> KFSAKRLPSTRLGTFLENRVNDFLRRQNHPESGEVTVRVVHASDKTVEVKPGMKARFVDSGEMAESFPYRTKALFAFEEIDGVDLCFFGMHVQEYGSDCPPPNQRRVYISYLDSVHFFRPKCLRTAVYHEILIGYLEYVKKLGYTTGHIWACPPSEGDDYIFHCHPPDQKIPKPKRLQEWYKKMLDKAVSERIVHDYKDIFKQATEDRLTSAKELPYFEGDFWPNVLEESIKELEQKTSKNKSSLSRGNKKKPGMPNVSNDLSQKLYATMEKHKEVFFVIRLIAGPAANSLPPIVDPDPLIPCDLMDGRDA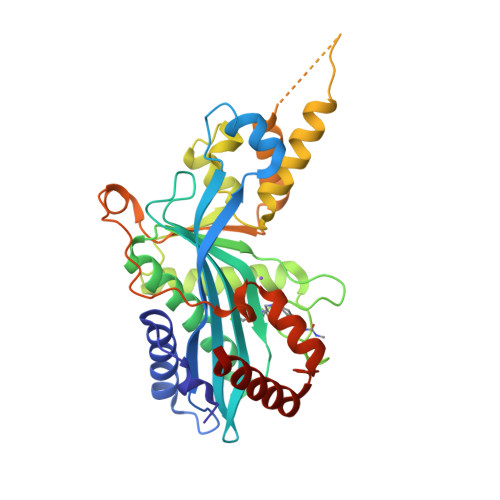FLTLARDRHLEFSSLRRAQWSTGCMLVELHTQSQDRF>GAMGSGNQTRALLDDQARHLLTEQERATMMYYLAQYRGGTISVEAMVMALFELLNTHAKFSLLSEVRSIISPQDLDRF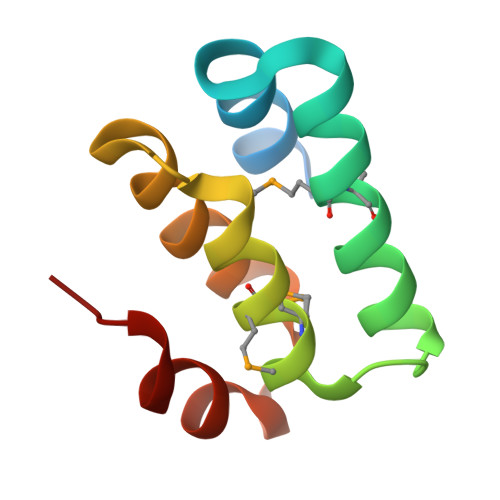DHLVLRR[6x]> AGVPFNTKYPYGPTSIADNQSEVTAMLKAEWEDWKSKRITSNGAGGYKRVQRDASTNYDTVSEGMGYGLLLAVCFNEQALFDDLYRYVKSHFNGNGLMHWHIDANNNVTSHDGGDGAATDADEDIALALIFADKQWGSSGAINYGQEARTLINNLYNHCVEHGSYVLKPGDRWGGSSVTNPSYFAPAWYKVYAQYTGDTRWNQVADKCYQIVEEVKKYNNGTGLVPDWCTASGTPASGQSYDYKYDA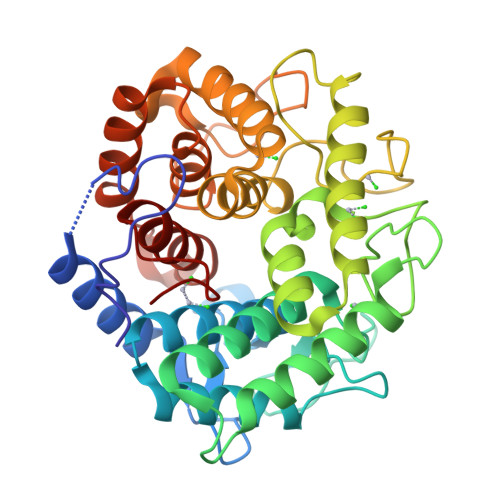TRYGWRTAVDYSWFGDQRAKANCDMLTKFFARDGAKGIVDGYTIQGSKISNNHNASFIGPVAAASMTGYDLNFAKELYRETVAVKDSEYYGYYGNSLRLLTLLYITGNFPNPLSDL> GSMVEATAQETDRPRFSFSIAAREGKARTGTIEMKRGVIRTPAFMPVGTAATVKALKPETVRATGADIILGNTYHLMLR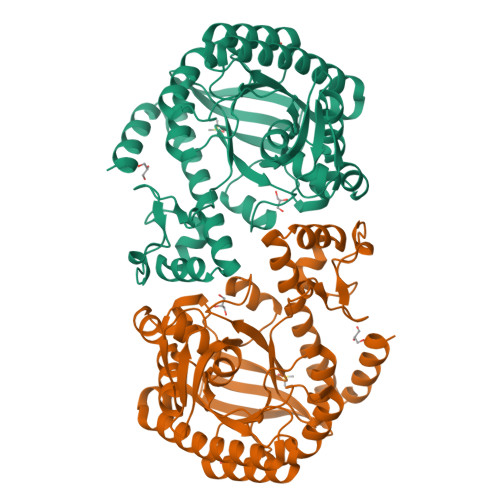PGAERIAKLGGLHSFMGWDRPILTDSGGYQVMSLSSLTKQSEEGVTFKSHLDGSRHMLSPERSIEIQHLLGSDIVMAFDECTPYPATPSRAASSMERSMRWAKRSRDAFDSRKEQAENAALFGIQQGSVFENLRQQSADALAEIGFDGYAVGGLAVGEGQDEMFRVLDFSVPMLPDDKPHYLMGVGKPDDIVGAVERGIDMFDCVLPTRSGRNGQAFTWDGPINIRNARFSEDLKPLDSECHCAVCQKWSRAYIHHLIRAGQILGAMLMTEHNIAFYQQLMQKIRDSISEGRFSQFAQDFRARYFARNS The icosahedral capsid contains 60 copies of a protomeric unit composed of four proteins, VP1-4. Enteroviruses are unique in harbouring a lipid molecule (pocket factor) within a pocket in the VP1 β-barrel, which lies below the surface of a deep depression encircling each fivefold axis, termed the canyon. The binding of such receptors can trigger pocket factor release and viral expansion, leading to externalization of the N-terminus of VP1 followed by VP4 to form a pore in the endo/lysosome membrane through which the genome is thought to be subsequently released. Here, we have determined three cryo-EM structures following mixing of CV-A10 Kowalik strain with KRM1: the CV-A10 mature virus, a disassembly intermediate A-particle and the mature virus in complex with KRM1.

The CVA-10 particle seen in the receptor complex is in the native (mature) conformation and the model comprises the same residues. Receptor binding has minimal impact on the capsid structure; structural superposition yields an RMSD of 0.5 Å for Cα atoms between mature virus and complexed-virus protomers. However, there are minor conformational rearrangements in some contact regions, most notably the C-terminus of VP3 and the VP2 EF loop. There is a noticeable reduction in the amount of bound pocket factor (to perhaps half the level seen in the mature virus particle). Residues 29–322 of KRM1 were modelled and two of the four glycosylation sites (N45 and N59) have well-defined density for the first glycans. KRM1 binds CV-A10 with a relatively large footprint (~1400 Å2) and the first two domains of KRM1 (KR and WSC) span the virus canyon, each making interactions with both the north and south rim. Although KRM1 dips into the canyon it does not reach the canyon floor. The KR domain engages at the narrow part of the canyon, contacting the C-terminus of VP3, EF loop of VP2, and the HI-loop of VP1 from a neighbouring protomer. Notably a loop spanning residues 98–102 in the KR domain, disordered in the high-resolution crystal structure, is ordered in the complex by a strong electrostatic interaction between Asp 102 at the tip of the loop with Arg 239 in the HI-loop of the adjacent CV-A10 protomer, whilst Tyr 105, Trp 106 and Tyr 108 in the same KR loop make weak interactions with Lys 140 of VP2 (Trp 106 stacking with the side chain stalk). The WSC domain of KRM1 binds the wider region of the canyon, interacting with the VP1 EF loop, VP2 EF loop, GH loop of VP1, VP3 GH loop, VP3 BC loop and the VP1 C-terminus from a neighbouring protomer. The CV-A10/KRM1 complex we report here demonstrates that relatively large non-Ig superfamily receptors can attach directly to the canyon and drive uncoating even without penetrating the canyon sufficiently to make direct interactions with the canyon floor.

> GDPVEDIIHDALSSTVRRAITSGQDVNTAAGTAPSSHRLETGRVPALQAAETGATSNATDENMIETRCVMNRNGVLEATISHFFSRSGLVGVVNLTDGGTDTTGYAVWDIDIMGFVQLRRKCEMFTYMRFNAEFTFVTTTENGEARPFMLQYMYVPPGAPKPTGRDAFQWQTATNPSVFVKLTDPPAQVSVPFMSPASAYQWFYDGYPTFGQHPETSNTTYGQCPNNMMGTFAVRVVSRVASQLKLQTRVYMKLKHVRAWIPRPIRSQPYLLKNFPNYDSSKITYSARDRASIKQANM;> SPSVEACGYSDRVAQLTVGNSSITTQEAANIVLAYGEWPEYCPDTDATAVDKPTRPDVSVNRFYTLDSKMWQENSTGWYWKFPDVLNKTGVFGQNAQFHYLYRSGFCLHVQCNASKFHQGALLVAVIPEFVLAGRGSNTKPNEAPHPGFNTTFPGTAGASFNDPYVLDSGVPLSQSLIYPHQWINLRTNNCATIIVPYINAVPFDSAINHSNFGLIVVPVSPLKYSSGATTAIPITVTIAPLNSEFGGLRQAVSQ;> GLPTELRPGTNQFLTTEDDTAAPILPGFSPTPSIHIPGEVRSLLELCRVETILEVNNTTDATGLNRLLIPVSAQNKADELCAAFMVDPGRIGPWQSTLVGQICRYYTQWSGSLKVTFMFTGSFMATGKMLIAYSPPGSAQPANRETAMLGTHVIWDFGLQSSVSLVIPWISNTHFRTAKTGGNYDYYTAGVVTLWYQTNYVVPPETPGEAYIIAMGAAQDNFTLKICKDTDEVTQQAVLQ;> MGAQVSSQRSGSHETGNVATGGSTINFTNINYYKDSYAASASRQDFTQDPKKFTQPVLDSIRELSAPLN;> ETGAPSPGLGPGPECFTANGADYRGTQNWTALQGGKPCLFWNETFQHPYNTLKYPNGEGGLGEHNYCRNPDGDVSPWCYVAEHEDGVYWKYCEIPACQMPGNLGCYKDHGNPPPLTGTSKTSNKLTIQTCISFCRSQRFKFAGMESGYACFCGNNPDYWKYGEAASTECNSVCFGDHTQPCGGDGRIILFDTLVGACGGNYSAMSSVVYSPDFPDTYATGRVCYWTIRVPGASHIHFSFPLFDIRDSADMVELLDGYTHRVLARFHGRSRPPLSFNVSLDFVILYFFSDRINQAQGFAVLYQAVKEEGSENLYFQGGSLPQERPAVNQTVAEVITEQANLSVSAARSSKVLYVITTSPSHPPQTVPGTHHHHHHHHHH>[2x]MHKEVKARYDEQMVLKKAALLYHFQPEQVTFLADAENYVYEYTDEKGSSYILKITHTIRRSSTYILGEMDWIRYLSQHGISVAKPVLSARGKDVEAIPDQAGGAFLLRVYEKAPGRKVTEADWNGQLFQALGAYTGRMHQTTKQYQVKDPRYKRQ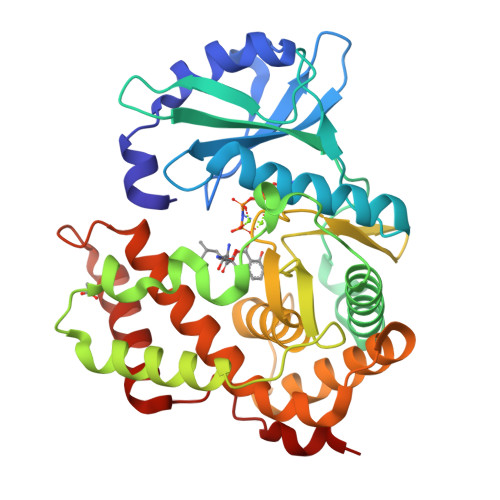EWYEEEQLKLETYIPSDQTVVLQRKDELMQKLHQLRISKDVYGLVHADLHHGNFHYHQGEIIAFDFDDCGYHWFINDISILLYNVLWYPVIPYEDKAEFTGEFMSHFLKGYRQENELDDAWLATIPDFLMLRHMLIYGLLHQAFDLRTLSADESAMLARFRKEIEDKTPITPFDFHQLTT> CTSIVAQNSAGQIIHGRNLDYDMTELLKNITIHVDFVRNGTIQYSGLTFALYNGVLTGQRPGEYSVSLNARYSGAYIDNILMEFYTKFKRPVS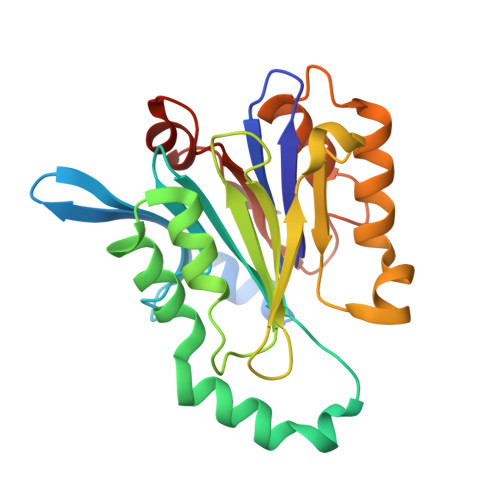FFIRDVLENQATYTEAVDAFSRTHLFSPSYIIVAGIKKNEGVVISRNRWSAANVYPLNVDANQWFLVETNFDNWKKQGDDRRITAIQKLKELGRRNFDEKSMVEVLSTVPVRNNLTVFSTVMVPGLPDSADYFRQSTWILP> MERKALVTGGSRGIGRAIAEALVARGYRVAIASRNPEEAAQSLGAVPLPTDLEKDDPKGLVKRALEALGGLHVLVHAAAVNVRKPALELSYEEWRRVLYLHLDVAFLLAQAAAPHMAEAGWGRVLFIGSVTTFTA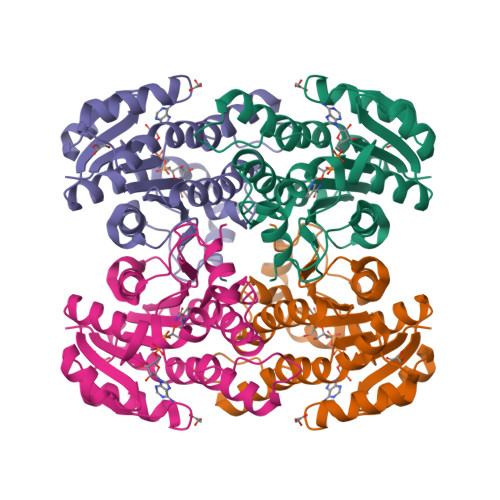GGPVPIPAYTTAKTALLGLTRALAKEWARLGIRVNLLCPGYVETEFTLPLRQNPELYEPITARIPMGRWARPEEIARVAAVLCGDEAEYLTGQAVAVDGGFLAY(9beta,13alpha)-3-hydroxyestra-1,3,5(10)-trien-17-one | C18 H22 O2 | 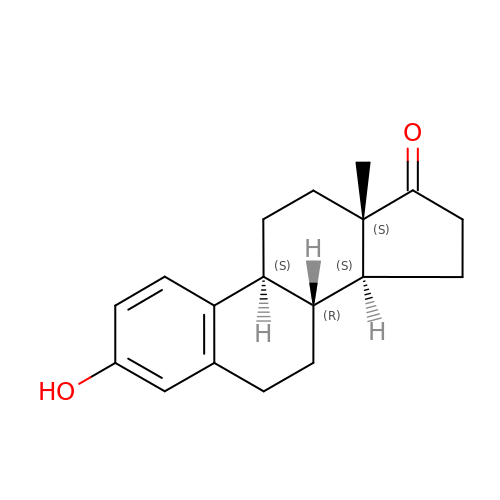DNXHEGUUPJUMQT-CBZIJGRNSA-N>GSGSTPNVDMVGWAYVDVKIVNTVADLESLTANDGMVAYVKGYYQPTNFALAKPYVGGGHRIYVASRAAENDGFLCINGWVLQIENNTVSPEHAGAKLNTPSFDSAIPIQKVLISGCKVRLNGLYHTSVPVYYNSNTTIEGTGELDCGFIKTTNNTLSLGNRTINGKIMNFDVDAIMVAIPRVGDWYAQNNHLSGFTLQYDSALPTKGIGLYAPLIALSTYKSILTKNTFEGIKSVDAWMCTWERVQASASSRSFIFGHTGTAWTPNNTTQTFIGCWATDAGLYGWDLNKMQGCTMISCGADFVGADGSPAKALFKIVYSNVTMVTCMNEHLHAQNFLYAEGSEVNISNFNGQAIYNKYKPATSSWNNNNSMFCVVSNSKVKLTGGSFGFAYNSSDPTQGANCSALAYVEGGSVFEVSPETTFAVPLEEIGISSLTAFTKLGVYYTTNASVDAYVKGVRYQDGAKFSGLVMDSYLSTSAKSLGNESITNLRGSLGNAVLVQSSTANATVANGFPSSGVPYLVQQWSSAAGNNSYNAQL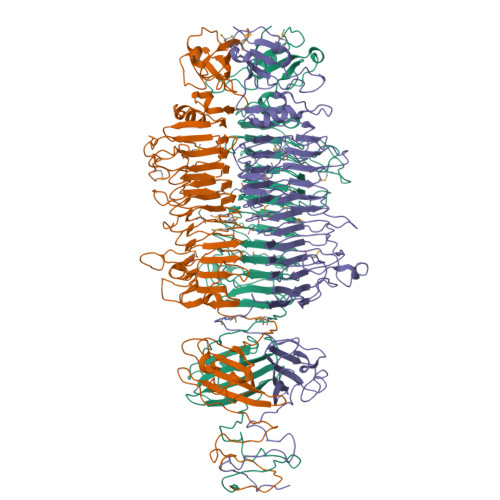AFAISSASATFWLRTGDYGQAYASWCRLYHYRDSLIPAATNTYDLGSSGSTFRNAYLQNAVTVVSDARKKSEVSELTEEELKCAVACGKLYRKYKLNDAIAEKGLENARYHFGVIAQEIMQCFTDYGLDWSKYGIITYDEWEDNTEEGIEAGNIYMVRYSELNCFVNAGIDYRLSLLE[3x]>IQTTAPPVKESSFVEKMKKTGRNIIVFYGSQTGTAEEFANRLSKDAHRYGMRGMSADPEEYDLADLSSLPEIDKSLVVFCMATYGEGDPTDNAQDFYDWLQETDVDLTGVKFAVFGLGNKTYEHFNAMGKYVDQRLEQLGAQRIFELGLGDDDGNLEEDFITWREQFWPAVCEFFGVEATGEESSIRQYELVVHEDMDVAKVYTGEMGRLKSYENQKPPFDAKNPFLAAVTANRKLNQGTERHLMHLELDISDSKIRYESGDHVAVYPANDSALVNQIGEILGADLDVIMSLNNLDEESNKKHPFPCPTTYRTALTYYLDITNPPRTNVLYELAQYASEPSEQEHLHKMASSSGEGKELYLSWVVEARRHILAILQDYPSLRPPIDHLCELLPRLQARYYSIASSSKVHPNSVHICAVAVEYEAKSGRVNKGVATSWLRAKEPAGENGGRALVPMFVRKSQFRLPFKSTTPVIMVGPGTGIAPFMGFIQERAWLREQGKEVGETLLYYGCRRSDEDYLYREELARFHKDGALTQLNVAFSREQAHKVYVQHLLKRDREHLWKLIHEGGAHIYVCGDARNMAKDVQNTFYDIVAEFGPMEHTQAVDYV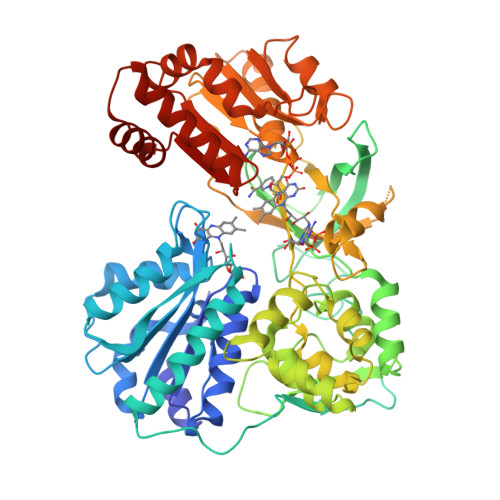KKLMTKGRYSLDV[2x]> MSLLLTLAKEYANLTKDKKSCKLLSQGTVSSYTTFKKWTTSRKEKNPSLRMRWAMGSKFPIMANREILEEAGIPEQWEGIDLWSKKDDVSKLGMVLASPAAITYWNFCGPGVDNSSVIKDVYKAKFMKKERWRETLWGPMNFELVGKQRRVVETQPVEIKLNQKEIKELTMWVLFEDEANLASKFIQENFSLVLSLRELYKGKAVNKDVAAFMIAHQFSPEKRFLPTFGPIRPERMELLHCLGGDFWKIEAVTAGSLNEEQKKRDVRAVARKICLRASVDLFTPAEKIRDYIASVTMRFGTVERTFEDVIRNSDDISAEVTLCKAALGCELGKSMSFGNLNLRKVSGEAETMEKTVYWGLKPIKYKCWRGEETFYCELRKVTCMFRRSEGLDWANIGPGSPEERRELLAMVMIFCRDGRFFESAPVNIDESFFRTRLNKEIPYQYVLLKWVRQSRDNLDALLSTRGLIPAHIGQFGKGMGIDGSSSSSMVYKGVMLSKTPIDIVESKEKHRLFLNDNIEAVTERGAMVASIMDLSEDNRETFNDVTFNHVDLAVLKDEKTAIIKIYRSLVERINTDDDGLPALIMGK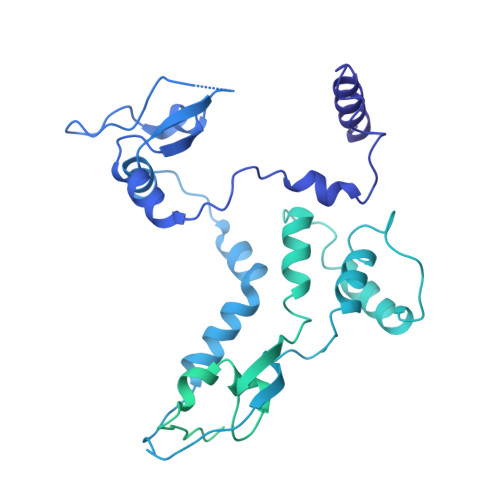RYLELYQLDEVKDAVGLIPKRMLGAYSYQARQLIQSQIKNDSYSLPEIIKLLPFCYSPPKKMLFDGTFHFKNQMYVRPGINTNLFSFSKTDKSKIYVNGSAVKIKLVLGDDEMDTSLAFVEGFQVCEYDPRAPLIPRRDLRLIGFGKKVRVFVGQGQEKTLVRTSSKRAASHDVSKNIRRMRLEV> MSSLRLVSSSTIQAANDNNDDSSQLIDLTVWDLIGLERESIQQGLLYHHPNQVDTPNQIQHLKHSLSSTLSFFPPFAGRLVITEYEDNTATCFIACNNAGALFVHAVAENTTISDILQPNKYVPPIVNSLFSLNGVKNREGTIQPLLVVQVTELVDGIFIGLTVNHVVADGKSFWLFVNSWAEISRGFQKPSKLPTLERWFLNDTDHPIRFSFSMEEEKKKFQSGQLTTRFFHFTRENIAHLKSKANGEVTLGNTERRISSLQALLAHVWRSVVRCERIDPQEVLYYILLIDARTRLIPPLEDDYFGNAADAGVVIMKAGELLEGGLGNVAWNMNKVISLNSDEKIKNRYKSWLRTPQLPSMGMHTTFASQLLIIANSPRFNVYGNDFGWGKPLAVRSSAENKRDCKIVLFAGAEEGSIDIEVCLPYEILEALGNDAEFLDNHSIG

Here we report a saponin acetyltransferase from Astragalus membranaceus. AmAT7-3 is discovered through a stepwise gene mining approach and characterized as the xylose C3′/C4′-O-acetyltransferse of astragaloside IV. AmAT7-3 is a rare multi-site acetyltransferase which acetylate large saponin molecules. We solved the crystal structures of AmAT7-3 and its variant A310G in complex with astragaloside IV, respectively.

To further elucidate how adjacent amino acids contributed to the conformation of the xylosyl group (Xyl) and regulated the regioselectivity of AmAT7-3, we analyzed the complex structure of AmAT7-3/astragaloside IV. In addition to the established critical role of H166, ten amino acids within 5 Å from the substrate were found to participate in building the internal structure of the active cavity. These amino acids include K407, R38, D311, A312, A310, L290, I34, I288, I374, and A376, which may play a decisive role in determining the substrate conformation. Unlike other acetyltransferases, the amino acids composing the β10 barrel (AADAG) in AmAT7-3 were relatively small in size, resulting in a larger active pocket to accommodate the saponin molecules such as astragaloside IV. Due to the relatively spacious pocket of AmAT7-3, we observed significant rotational motion of the xylosyl sugar ring throughout the MD simulation. Based on the rotation angles, we segregated the substrate into two major conformations using a 75-degree threshold. In conformation-1, the O3′ and O4′ sites formed hydrogen bonds with K407 and H166, respectively. This H-bonding constrained the substrate, positioning the O3′ site in close proximity to Cx, implying a potential site for selective acetylation. Our calculations showed that the reaction was initiated by the proton transfer from sugar O atom to His166, which was coupled to the nucleophilic attack of sugar O onto the acyl Cx, leading to the formation of a tetrahedral intermediate.>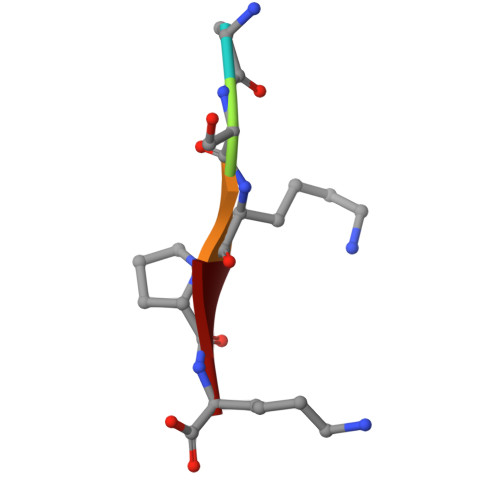 ASKPK In yeast, the evolutionarily conserved GID E3 ligase mediates glucose-induced degradation of fructose-1,6-bisphosphatase (Fbp1), malate dehydrogenase (Mdh2), and other gluconeogenic enzymes. “GID” is a collection of E3 ligase complexes; a core scaffold, RING-type catalytic core, and a supramolecular assembly module together with interchangeable substrate receptors select targets for ubiquitylation. Here, we structurally and biochemically characterize Gid12 as a modulator of the GID E3 ligase complex. Our collection of cryo-EM reconstructions shows that Gid12 forms an extensive interface sealing the substrate receptor Gid4 onto the scaffold, and remodeling the degron binding site.

To gain insights into potential functions of Gid12, we obtained cryo-EM reconstructions for Gid12 bound to the substrate-receptor and scaffolding (SRS) module (a Gid12-Gid4-Gid5-Gid1-Gid8 complex, referred to as Gid12-SRS), to GIDSR4 (referred to as Gid12-GIDSR4), and to Chelator-GIDSR4 (referred to as Gid12-Chelator-GIDSR4) at 3.3, 9.8, and 19.4 Å resolution, respectively. Thus, we built coordinates for Gid12-SRS, and generated atomic models of Gid12-GIDSR4 and Gid12-Chelator-GIDSR4 by docking them with Gid12-SRS and the respective prior structures of GIDSR4 and Chelator-GIDSR4. In agreement with the biochemical data, Gid12 primarily contacts Gid4, and also Gid5. Gid12 emanates from and extends this groove, to wrap ≈305° around Gid4. Three insertions (Ins4, Ins4-5 and Ins5-6) form helical structures that pack either against the sides of the propeller or between blades, while an insertion in the third blade of Gid12 (Ins3) forms a meandering loop that plugs the central pore on the bottom face of the propeller. Gid12’s interactions with Gid4 and Gid5 bury more than 2400 Å2 of surface area. The Gid12-Gid5 interaction primarily involves the edges of blades 1 and 7 on the side of the Gid12 propeller binding a ≈ 30-residue Gid5 region that was disordered in prior structures and is presumably stabilized in the complex. Gid12 interacts across a diagonal around all eight strands in the Gid4 β-barrel, from the N-terminal tip of strand 4 at one edge of the cylinder, nearly the entire length of strands 1 and 8 at the center of the interaction, to the N-terminal tip of strand 5 at the other edge of the cylinder. Gid12 extracts Gid4’s L2-loop, such that Leu172 and surrounding residues faces outside the central cylinder, and bind a pocket at the junction between Gid12’s blades 7 and 1.

> MSEYMDDVDREFINCLFPSYLLQQPVAYDLWILYLQHRKLFHKLKNTNLINADENPTGVGMGRTKLTALTRKEIWSKLMNLGVLGTISFEAVNDDYLIQVYKYFYPDVNDFTLRFGVKDSNKNSVRVMKASSDMRKNAQELLEPVLSEREMALNSNTSLENDRNDDDDDDDDDDDDDDDDDDDDDESDLESLEGEVDTDTDDNNEGDGSDNHEEGGEEGSRGADADVSSAQQRAERVADPWIYQRSRSAINIETESRNLWDTSDKNSGLQYYPPDQSPSSSFSSPRVSSGNDKNDNEATNVLSNSGSKKKNSMIPDIYKILGYFLPSRWQAQPNNSLQLSQDGITHLQPNPDYHSYMTYERSSASSASTRNRLRTSFENSGKVDFAVTWANKSLPDNKLTIFYYEIKVLSVTSTESAENSNIVIGYKLVENELMEATTKKSVSRSSVAGSSSSLGGSNNMSSNRVPSTSFTMEGTQRRDYIYEGGVSAMSLNVDGSINKCQKYGFDLNVFGYCGFDGLITNSTEQSKEYAKPFGRDDVIGCGINFIDGSIFFTKNGIHLGNAFTDLNDLEFVPYVALRPGNSIKTNFGLNEDFVFDIIGYQDKWKSLAYEHICRGRQMDVSIEEFDSDESEEDETENGPEENKSTNVNEDLMDIDQEDGAAGNKDTKKLNDEKDNNLKFLLGEDNRFIDGKLVRPDVNNINNLSVDDGSLPNTLNVMINDYLIHEGLVDVAKGFLKDLQKDAVNVNGQHSESKDVIRHNERQIMKEERMVKIRQELRYLINKGQISKCINYIDNEIPDLLKNNLELVFELKLANYLVMIKKSSSKDDDEIENLILKGQELSNEFIYDTKIPQSLRDRFSGQLSNVSALLAYSNPLVEAPKEISGYLSDEYLQERLFQVSNNTILTFLHKDSECALENVISNTRAMLSTLLEYNAFGSTNSSDPRYYKAINFDEDVLNL;> MINNPKVDSVAEKPKAVTSKQSEQAASPEPTPAPPVSRNQYPITFNLTSTAPFHLHDRHRYLQEQDLYKCASRDSLSSLQQLAHTPNGSTRKKYIVEDQSPYSSENPVIVTSSYNHTVCTNYLRPRMQFTGYQISGYKRYQVTVNLKTVDLPKKDCTSLSPHLSGFLSIRGLTNQHPEISTYFEAYAVNHKELGFLSSSWKDEPVLNEFKATDQTDLEHWINFPSFRQLFLMSQKNGLNSTDDNGTTNAAKKLPPQQLPTTPSADAGNISRIFSQEKQFDNYLNERFIFMKWKEKFLVPDALLMEGVDGASYDGFYYIVHDQVTGNIQGFYYHQDAEKFQQLELVPSLKNKVESSDCSFEFA;> MTVAYSLENLKKISNSLVGDQLAKVDYFLAPKCQIFQCLLSIEQSDGVELKNAKLDLLYTLLHLEPQQRDIVGTYYFDIVSAIYKSMSLASSFTKNNSSTNYKYIKLLNLCAGVYPNCGFPDLQYLQNGFIQLVNHKFLRSKCKIDEVVTIIELLKLFLLVDEKNCSDFNKSKFMEEEREVTETSHYQDFKMAESLEHIIVKISSKYLDQISLKYIVRLKVSRPASPSSVKNDPFDNKGVDCTRAIPKKINISNMYDSSLLSLALLLYLRYHYMIPGDRKLRNDATFKMFVLGLLKSNDVNIRCVALKFLLQPYFTEDKKWEDTRTLEKILPYLVKSFNYDPLPWWFDPFDMLDSLIVLYNEITPMNNPVLTTLAHTNVIFCILSRFAQCLSLPQHNEATLKTTTKFIKICASFAASDEKYRLLLLNDTLLLNHLEYGLESHITLIQDFISLKDEIKETTTESHSMCLPPIYDHDFVAAWLLLLKSFSRSVSALRTTLKRNKIAQLLLQILSKTYTLTKECYFAGQDFMKPEIMIMGITLGSICNFVVEFSNLQSFMLRNGIIDIIEKMLTDPLFNSKKAWDDNEDERRIALQGIPVHEVKANSLWVLRHLMYNCQNEEKFQLLAKIPMNLILDFINDPCWAVQAQCFQLLRNLTCNSRKIVNILLEKFKDVEYKIDPQTGNKISIGSTYLFEFLAKKMRLLNPLDTQQKKAMEGILYIIVNLAAVNENKKQLVIEQDEILNIMSEILVETTTDSSSYGNDSNLKLACLWVLNNLLWNSSVSHYTQYAIENGLEPGHSPSDSENPQSTVTIGYNESVAGGYSRGKYYDEPDGDDSSSNANDDEDDDNDEGDDEGDEFVRTPAAKGSTSNVQVTRATVERCRKLVEVGLYDLVRKNITDESLSVREKARTLLYHMDLLLKVK;> MTISTLSNETTKSGSCSGQGKNGGKDFTYGKKCFTKEEWKEQVAKYSAMGELYANKTIHYPLKIQPNSSGGSQDEGFATIQTTPIEPTLPRLLLNYFVSMAYEDSSIRMAKELGFIRNNKDIAVFNDLYKIKERFHIKHLIKLGRINEAMEEINSIFGLEVLEETFNATGSYTGRTDRQQQQQQQQFDIDGDLHFKLLLLNLIEMIRSHHQQENITKDSNDFILNLIQYSQNKLAIKASSSVKKMQELELAMTLLLFPLSDSADSGSIKLPKSLQNLYSISLRSKIADLVNEKLLKFIHPRIQFEISNNNSKFPDLLNSDKKIITQNFTVYNNNLVNGSNGTKITHISSDQPINEKMSSNEVTAAANSVWLNQRDGNVGTGSAATTFHNLENKNYWNQTSELLSSSNGKEKGLEFNNYYSSEFPYEPRLTQIMKLWCWCENQLHHNQIGVPRVEN;> MATGRIQFAVSTPCNTKGKPSGYRLFEFKNDRLALVPSERGCTKVDVNANIQAFCYLRPNGRDTSISPDATHILDSCDYMVLAKSNGFIEIISNYQYKIKNGLRLAPSYILRCTPEDFESNFFSDYMIAGLEYSQGLLYCCMCSGRIYVFVMNLPTDYIQYKNMYNPMFPDCFFKVHHDNNTTHSSEEEKLFEGSTRYTGRSCSKHICYFLLPIEPSHLRSSPVVSSFCNMYQGLPIYRPSMYLHIERGISTFHINPLDRFCFMTVSPRSPLFIRKIILPLTYVTFLSTFISLKNSIQGDTCGEILSWDNVAQQNGFGSLFSWISNKFTFDTDIINSTIWDDIVKYSGTGMLDSGIVWKQRQGHAKDDIYELFHTQDMLGSSRRNSSFSTASSEPRPLSRRRRESFQALTRDAFRERMDVPCSTKWELDSFIRGLRRNTFMVDFEIVEKISHRNGNDGVNEDDNTTDESDETMTSFLTDNYKKMDIVCIDHFVTLSAFRPRYYDEPIIKIDSLSNKNGSENGTNEEEWAESQMKVDGQVIDDETAQFKQALGNLCSFKKLFMLDDSLCFILDTHGVLLINRFEIKNTKNLLRNSKDTIRIIPHDFGLINDTIVIINDIDVGTDNVCALTFHLVVTSMAGEITVLKGEFFKNCRLGRIKLCDSLKLNRKDRFVDKLALIDYDGLNAQKRRLDYDEKDLYTFIVKKVKRD>[2x]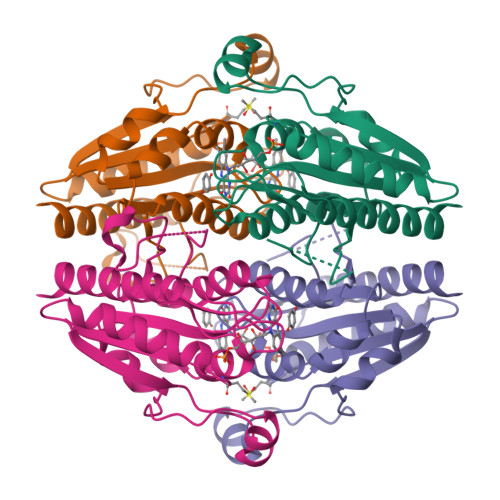AKVLVLYYSMYGHIETMARAVAEGASKVDGAEVVVKRVPETMPPQLFEKAGGKTQTAPVATPQELADYDAIIFGTPTRFGNMSGQMRTFLDQTGGLWASGALYGKLASVFSSTGTGGGQEQTITSTWTTLAHHGMVIVPIGYAAQELFDVSQVRGGTPYGATTIAGGDGSRQPSQEELSIARYQGEYVAGLAVKLNG>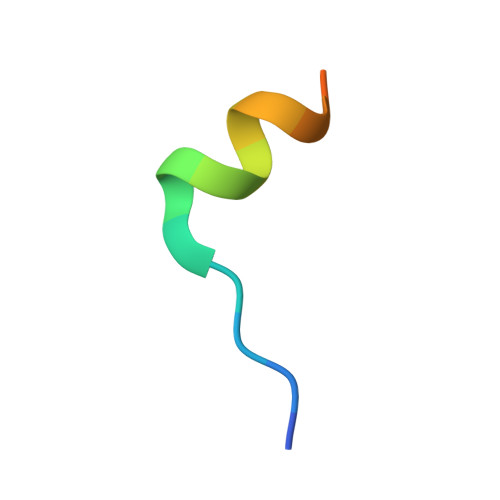 RIIYDRKFLMECRNSPV>[6x]MFGYFYNSSFRRYATLMGDLFSNIQIKRQLESGDKFIRVPITYASKEHFMMKLNKWTSINSQEDVAKVETILPRINLHLVDFSYNAPFKTNILNQNLLQKGATSVVSQYNPSPIKMI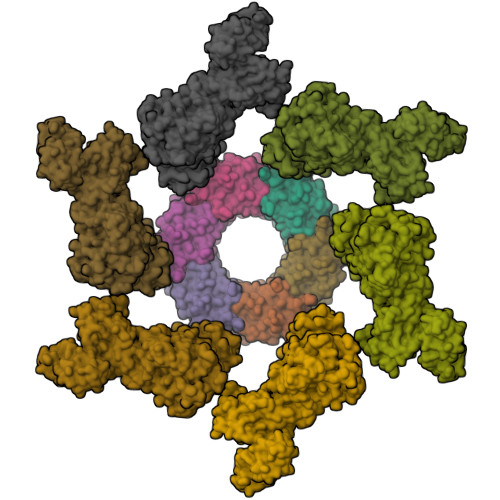YELSIFTRYEDDMFQIVEQILPYFQPHFNTTMYEQFGNDIPFKRDIKIVLMSAAIDEAIDGDNLSRRRIEWSLTFEVNGWMYPPVDDAEGLIRTTYTDFHANTRDLPDGEGVFESVDSEVVPRDIDPEDWDGTVKQTFTSNVNRPTPPEPPGPRT;>[6x]MTLLSPGIELKETTVQSTVVNNSTGTAALAGKFQWGPAFQIKQVTNEVDLVNTFGQPTAETADYFMSAMNFLQYGNDLRVVRAVDRDTAKNSSPIAGNIEYTISTPGSNYAVGDKITVKYVSDDIETEGKITEVDADGKIKKINIPTAKIIAKAKEVGEYPTLGSNWTAEISSSSSGLAAVITLGKIITDSGILLAEIENAEAAMTAVDFQANLKKYGIPGVVALYPGELGDKIEIEIVSKADYAKGASALLPIYPGGGTRASTAKAVFGYGPQTDSQYAIIVRRNDAIVQSVVLSTKRGGKDIYDSNIYIDDFFAKGGSEYIFATAQNWPEGFSGILTLSGGLSSNAEVTAGDLMEAWDFFADRESVDVQLFIAGSCAGESLETASTVQKHVVSIGDVRQDCLVLCSPPRETVVGIPVTRAVDNLVNWRTAAGSYTDNNFNISSTYAAIDGNYKYQYDKYNDVNRWVPLAADIAGLCARTDNVSQTWMSPAGYNRGQILNVIKLAIETPQAQRDRLYQEAINPVTGTGGDGYVLYGDKTATSVPSPFDRINVRRLFNMLKTNIGRSSKYRLFELNNAFTRSSFRTETAQYLQGNKALGGIYEYRVVCDTTNNTPSVIDRNEFVATFYIQPARSINYITLNFVATATGADFDELTGLAG>[6x]DQDKIEALSSKVQQLERSIGLKDLAMADLEQKVLEMEASTYDGVFIWKISDFARKRQEAVAGRIPAIF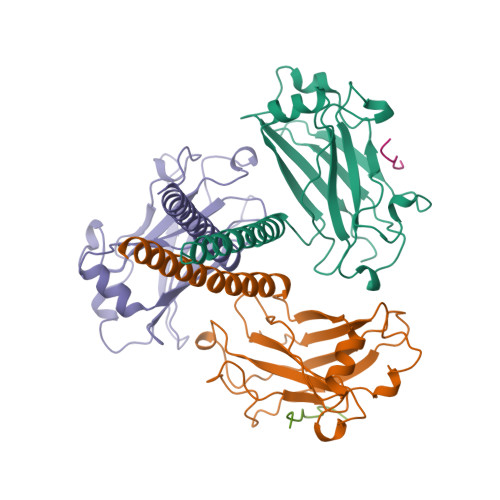SPAFYTSRYGYKMCLRIYLNGDGTGRGTHLSLFFVVMKGPNDALLRWPFNQKVTLMLLDQNNREHVIDAFRPDVTSSSFQRPVNDMNIASGCPLFCPVSKMEAKNSYVRDDAIFIKAIVDLTGL;>GQVPFSKEEC[2x]CD200 is a widely distributed membrane glycoprotein that regulates myeloid cell activity through its interaction with an inhibitory receptor (CD200R). CD200R is a member of a “paired receptor” family as in addition to this inhibitory receptor there is one very closely related gene with activating potential in humans and several in mice (Akkaya and Barclay, 2010; Wright et al., 2003). We report X-ray crystallography structures for the inhibitory CD200R, the activating receptor CD200RLa, and a complex between CD200R and CD200.

The structure of CD200R was solved by molecular replacement using the coordinates of CD200RLa as a search model. CD200R and CD200RLa contain typical Ig-like domains consisting of an NH2-terminal V-like domain followed by a smaller C2-like domain. The first NH2-terminal residue for which electron density was observed is P15 in CD200R and Q18 for CD200RLa. The absence of electron density for the potentially glycosylated NH2-terminal region suggests this region is flexible and able to adopt different conformations. Intrasheet disulfides are found between beta strand C′ and the C″D loop in the V-like domain and between beta strands D and E in the C2-like domain. Superposition of the V-like domains (residues 17–126) of CD200R alone and in complex with CD200 supports the earlier suggestion that the NH2-terminal region of CD200R is flexible; a rotation of the main chain around residue 17 results in residues 15-16 moving from the front GFC face (which would impede binding to CD200) to the back BED face, exposing the CD200 binding face. Other than the NH2 terminus, there are no significant changes to the interacting face of CD200R upon binding. Conformational differences between the bound and unbound CD200R are seen in the BC loop (residues 37–41), DE loop (residues 82–87), and to a lesser extent in the EF loop (residues 93–94). These loops are not involved in the interaction with CD200, and these differences are due to the different packing of the molecules within the crystals and also reflect the plasticity of these loops.

> TDKNQTTQNNSSSPLTQVNTTVSVQIGTKALLCCFSIPLTKAVLITWIIKLRGLPSCTIAYKVDTKTNETSCLGRNITWASTPDHSPELQISAVTLQHEGTYTCETVTPEGNFEKNYDLQVLVPPEVTYFPEKNRSAVCEAMAGKPAAQISWSPDGDCVTTSESHSNGTVTVRSTCHWEQNNVSDVSCIVSHLTGNQSLSIELGRGGSTRHHHHHH>EEPSDLEELEQFAKTFKQRRIKLGFTQGDVGLAM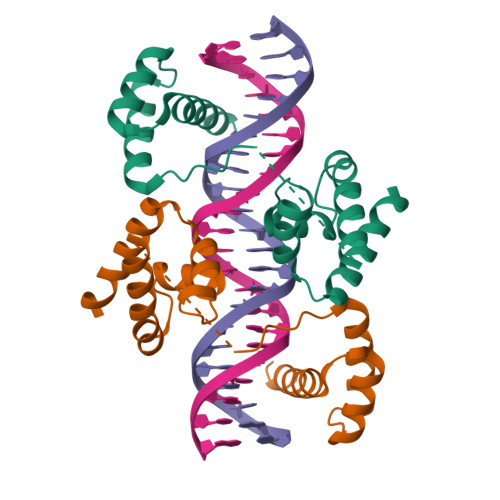GKLYGNDFSQTTISRFEALNLSFKNMSKLKPLLEKWLNDAENLSSDSSLSSPSALNSPGIEGLSRRRKKRTSIETNIRVALEKSFLENQKPTSEEITMIADQLNMEKEVIRVWFSNRRQKEKRIN[2x]> MPYNDIQHNFLKAMSDKFAEKPESTATEFYTYGGIAQKGGMRKREFIAEASKIVDSRVNSTPAYNPDAGMPQGQRYLMPYMMNHTDIMVNADDLHWINNAAMQQAWDDMKRGIVLGLDDAHGLLEARLGKEVTPDTISNYMEVLNHALPGGAVIQEHMVETKPMLVNDSYAKIFSGDDDLVDSVDRRFILDINKEFAAGYDKPGEQADQLKDAIGKKIWQILWMPTVVARQTDGGTMFRWVGMQVGMTMINAYKLCAGESVTGEFAYYAKHAAVVQLSNYMPVKRARSHNEPGGMPLGINADSTRSPALFPNDPIRAELESIAVAAMVYDQLWFGTYMSGGVGFTQYASATYTDNILEDFCYKGCEIGLDYAGGKMASIKGDKLNMDILEEIIRAENDYALTQYEAYPTVAESHFGGSVRACCAAAGCGSAVACATGLAQPALSAWSLSMLGHYERVGRLGFFGYDL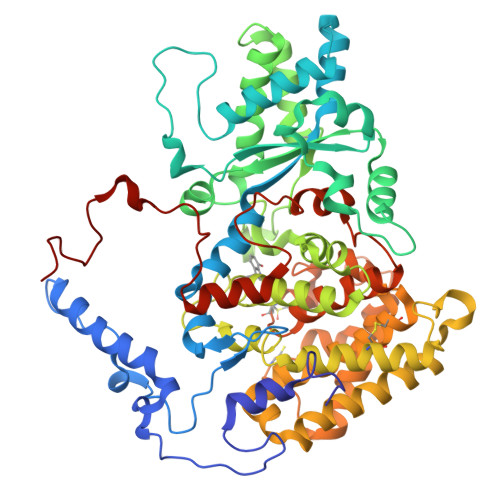QDQCTACGSYSYQSDEGMPFEMRGVNYPNYAMNVGHQSAYAGLVAGAHSANHDAWVLSPLWKVAFSDRDLPFDRGYVTREYGLGANREYTKVAGERDLIIAGHYGREPGAKL>[4x]MDSLDQCIVNACKNSWDKSYLAGTPNKDNCSGFVQSVAAELGVPMPRGNANAMVDGLEQSWTKLASGAEAAQKAAQGFLVIAGLKGRTYGHV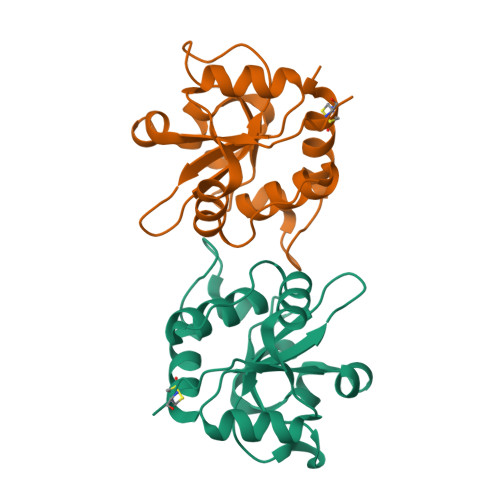AVVISGPLYRQKYPMCWSGSIAGAVGQSQGLKSVGQVWNRTDRDRLNYYVYSLASCSLPRASLEHHHHHH> AQRRKEREELAQ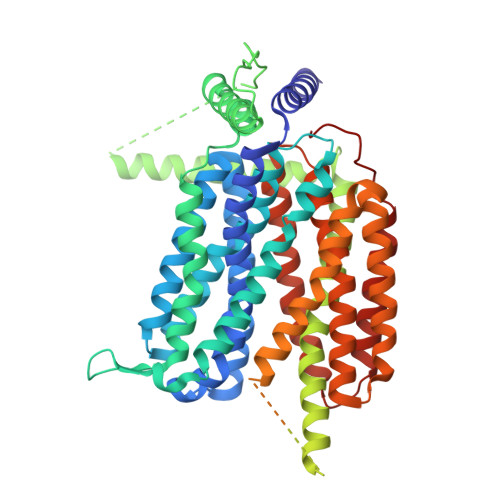QYEAILRECGHGRFQWTLYFVLGLALMADGVEVFVVGFVLPSAEKDMCLSDSNKGMLGLIVYLGMMVGAFLWGGLADRLGRRQCLLISLSVNSVFAFFSSFVQGYGTFLFCRLLSGVGIGGSIPIVFSYFSEFLAQEKRGEHLSWLCMFWMIGGVYAAAMAWAIIPHYGWSFQMGSAYQFHSWRVFVLVCAFPSVFAIGALTTQPESPRFFLENGKHDEAWMVLKQVHDTNMRAKGHPERVFSVTHIKTIHQEDELIEIQSDTGTWYQRWGVRALSLGGQVWGNFLSCFGPEYRRITLMMMGVWFTMSFSYYGLTVWFPDMIRHLQAVDYASRTKVFPGERVEHVTFNFTLENQIHRGGQYFNDKFIGLRLKSVSFEDSLFEECYFEDVTSSNTFFRNCTFINTVFYNTDLFEYKFVNSRLINSTFLHNKEGCPLDVTGTGEGAYMVYFVSFLGTLAVLPGNIVSALLMDKIGRLRMLAGSSVMSCVSCFFLSFGNSESAMIALLCLFGGVSIASWNALDVLTVELYPSDKRTTAFGFLNALCKLAAVLGISIFTSFVGITKAAPILFASAALALGSSLALKLPETRGQVLQ> DFVIPPINLPENSRGPFPQELVRIRSDRDKNLSLRYSVTGPGADQPPTGIFIINPISGQLSVTKPLDRELIARFHLRAHAVDINGNQVENPIDIVINVIDMNDNRPEFLHQVWNGSVPEGSKPGTYVMTVTAIDADDP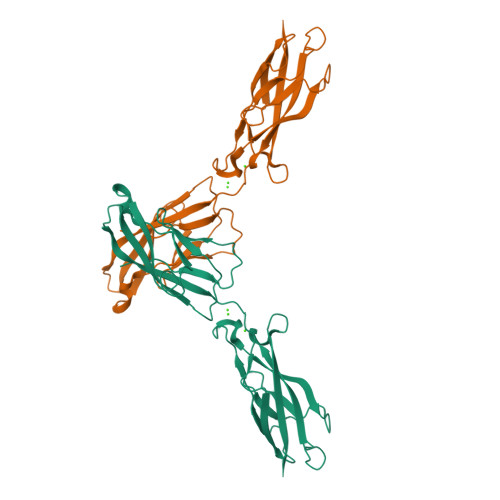NALNGMLRYRILSQAPSTPSPNMFTINNETGDIITVAAGLDREKVQQYTLIIQATDMEGNPTYGLSNTATAVITVTD> MTFLIKRETQVDQILRDIRAVVNQMVP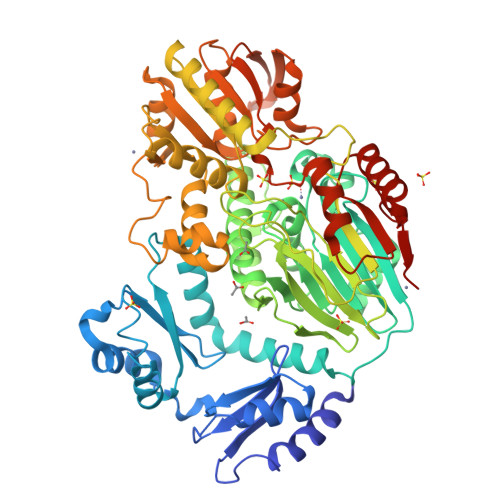KEAKITEIEFEGPELVIYVKNPEAIMKDGELIKDLAKVLKKRISVRPDPEVLLPPEEAEKLIFEIVPKEAEITNIAFDPSVGEVLIEAKKPGLVIGKNGETLRLITQKVKWAPKVVRTPPLQSQTIYSIRQILQTESKDRRKFLRQVGRNIYRKPEYKSRWIRITGLGGFREVGRSALLVQTDESFVLVDFGVNVAMLNDPYKAFPHFDAPEFQYVLREGLLDAIIITHAHLDHCGMLPYLFRYNLFDGPIYTTPPTRDLMVLLQKDFIEIQQSNGQDPLYRPRDIKEVIKHTITLDYGEVRDISPDIRLTLHNAGHILGSAIVHLHIGNGLHNIAITGDFKFIPTRLLEPANAKFPRLETLVMESTYGGANDIQMPREEAEKRLIEVIHNTIKRGGKVLIPAMAVGRAQEVMMVLEEYARIGGIEVPIYLDGMIWEATAIHTAYPEYLSRRLREQIFKEGYNPFLSEIFHPVANSRERQDIIDSNEPAIIIASSGMLVGGPSVEYFKQLAPDPKNSIIFVSYQAEGTLGRQVQSGIREIPMVGEEGRTEVIKVNMEVHTIDGFSGHADRRELMNYVAKVRPRPERIITVHGEPQKCLDLATSIHRKFGISTRAPNNLDTIRLR>MDIEFTTSAASQASLPRGRRTARPSGDDRELAILATAENLLEDRPLADISVDDLAKGAGISRPTFYFYFPSKEAVLLTLLDRVVNQADMALQTLAENPADTDRENMWRTGINVFFETFGSHKAVTRAGQAARATSVEVAELWSTFMQKWIAYTAAVIDAERDRGAAPRTLPAHELATALNLMNERTLFASFAGEQPSVPEARVLDTLVHIWVTSIYGENR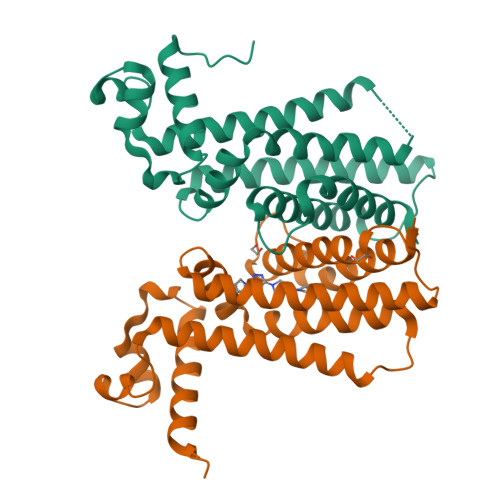GSHHHHHH[4x]>MGGNPEFVKFPEKYEQIFTHYDTANRANQTQLAKFYANEIAAESYKKGEEAAPGSIVIMEIYAPKKDAEGKIQSGED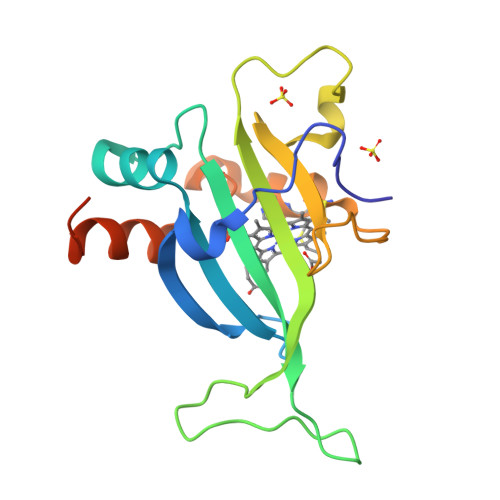GLFVIDKLAAIAVMEKRNDWGSAFKADDRSGNWGFALYDPEGKAKDNDLTCAQCHNPLQKQDNLFSFQKLVDYVKAHKLAAALELEHHHHHH[3x]>FACKTANGTAIPIGGGSANVYVNLAPAVNVGQNLVVDLSTQIFCHNDYPETITDYVTLQRGSAYGGVLSSFSGTVKYNGSSYPFPTTSETPRVVYNSRTDKPWPVALYLTPVSSAGGVAIKAGSLIAVLILRQTNNYNSDDFQFVW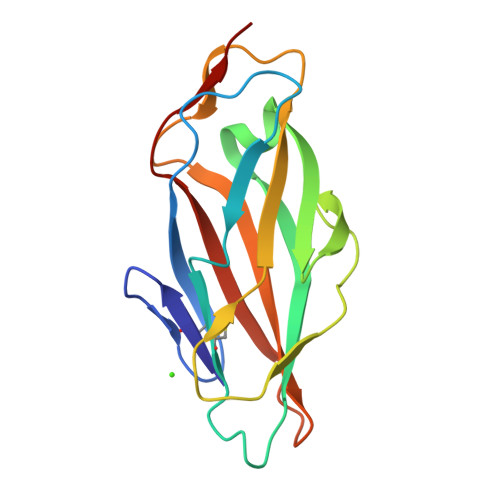NIYANNDVVVPTG[4x]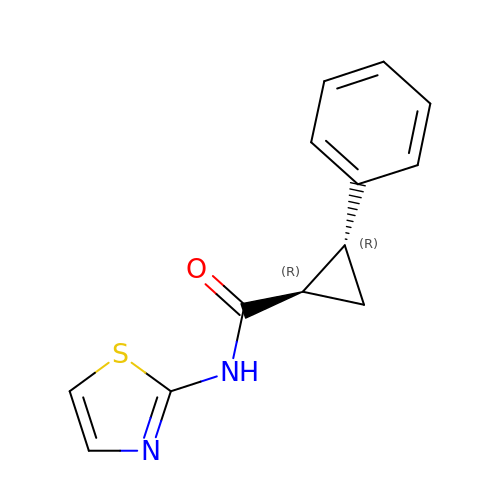(1~{R},2~{R})-2-phenyl-~{N}-(1,3-thiazol-2-yl)cyclopropane-1-carboxamide | C13 H12 N2 O S | ZOOMNALRJFPRHO-WDEREUQCSA-N>[3x]HHFEAYSLSDNDYDGIKKLLQQLFLKAPVNTAELTDLLIQQNHIGSVIKQTDVSEDSNDDMDEDEVFGFISLLNLTERKGTQCVEQIQELVLRFCEKNCEKSMVEQLDKFLNDTTKPVGLLLSERFINVPPQIALPMYQQLQKELAGAHRTNKPCGKCYFYLLISKTFVEAGKNNSKKKPSNKKKAALMFANAEEEF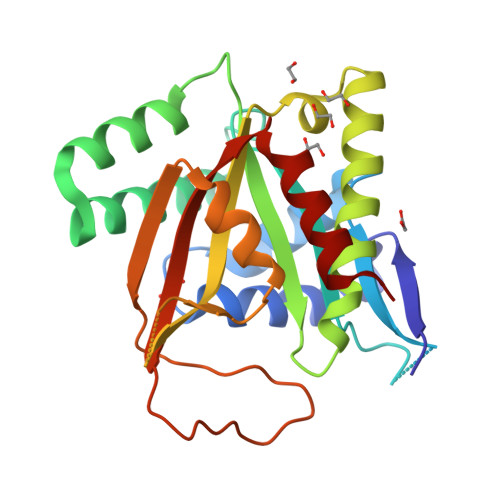FYEKAILKFNYSVQEESDTCLGGKWSFDDVPMTPLRTVMLIPGDKMNEIMDKLKEYLSV The Cry48Aa/Tpp49Aa pair is produced by a number of L. sphaericus strains and is composed of Cry48Aa, a 135-kDa protein belonging to the 3-domain family of Crystal (Cry) proteins, and Tpp49Aa, a 53 kDa protein belonging to the family of Toxin_10 pesticidal proteins (Tpp). Mosquito toxicity bioassays have revealed that both components in combination are required for activity against Culex quinquefasciatus larvae. Within each Tpp49Aa1 monomer, two distinct domains exist: an N-terminal lectin-like head domain covering residues 49–214 and a C-terminal putative pore-forming domain (PFD) covering residues 215–464. The final model of Tpp49Aa1 revealed the presence of a homodimer forming an “X” structure with a large intermolecular interface, similar to that described for natural heterodimeric crystals of Tpp1Aa2/Tpp2Aa2.

To do so, pH 11 buffer was injected into the vacuum chamber of the SPB/SFX beamline, allowing mixing with the natural Tpp49Aa1 crystals prior to data collection. In total, 707,992 diffraction patterns were collected from which 426,506 could be indexed in space group P212121, (a ~ 80.12; b ~ 83.22; c ~ 156.49 Å; α = β = γ = 90, highlighting an increase in unit-cell dimensions in comparison to the pH 7 dataset). Manual building and refinement from the ensembled diffraction data led to a model with Rwork/Rfree of 0.177/0.199 at 1.75 Å resolution. The pH 7 and pH 11 structures align closely, displaying an all-atom RMSD of 0.487 Å. As in the Tpp1Aa2/Tpp2Aa2 structure, an increase in pH from 7 to 11 is estimated to alter the net charge of Tpp49Aa1 from −6.518 to −47.822 e, suggesting that alkalinity will destabilize the crystal by negative electrostatic repulsion. Overall, the binding energy of all eight crystal contacts (excluding the dimer interface) increases by 1.8 kcal mol−1, indicating a weaker affinity. Despite this, the binding energy of the dimer interface decreases (pH 7 = −11.1, pH 11 = −11.9 kcal mol−1), indicating an increase in affinity. This may suggest that, during dissolution, contacts between individual dimers dissociate prior to the dimers themselves. The most notable changes include loss of hydrogen bonds Asn51[ND2]-Asn350[OD1] and Asn51[ND2]-Asp347[O] of both monomers at the dimer interface. Given the proximity of these interactions to the cleavage site (Phe48) of the N-terminal propeptide, we hypothesize that loss of these hydrogen bonds would increase accessibility of the propeptide to proteases.

>[2x]NLNLPEQSTRFQTIASIHSNNCSFEILNNDPGYIYGDSVDGECRIAVAHRELGNGLERTGDDRFLFIFYALDNNNFIIANRHDGFVLQFLIANGQGVIVSREYQPNIHQEFTIQSINSDTFRLHSRDTNTFATVCWAQFNSWTKIVSRVDNPGAPNANLKHRSLLTDINMPQLPSLTPLQPLPRLTELEDGGLSPAQAPRAIIGRTLIPCLFVNDPVLRLENRIKQSPYYVLEHRQYWHRIWTDIFTAGERREYREVTGINNNAQNDMNKMINITIGADGPNRLRFGNLSTPFRQQIIDNSNTLGSFANTNYGTRTDIVNVFNSEFHQVRYARFVKAYEYRLTRADGSQVGTPWVVLDRKEMDLRTYPHNMAITLENVKIDNADNSYDLSIWKTPLKLKDGKIIIENHENSKPYYN> QDCGLPPDVPNAQPALEGRTSFPEDTVITYKCEESFVKIPGEKDSVICLKGSQWSDIEEFCNRSQDCGLPPDVPNAQPALEGRTSFPEDTVITYKCEESFVKIPGEKDSVICLKGSQWSDIEEFCNRSCEVPTRLNSASLKQPYITQNYFPVGTVVEYECRPGYRREPSLS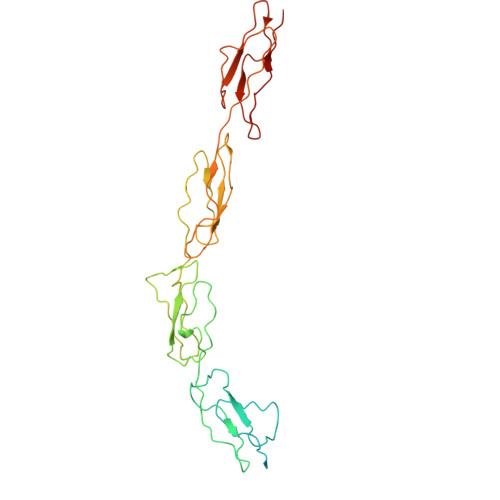PKLTCLQNLKWSTAVEFCKKKSCPNPGEIRNGQIDVPGGILFGATISFSCNTGYKLFGSTSSFCLISGSSVQWSDPLPECREIYCPAPPQIDNGIIQGERDHYGYRQSVTYACNKGFTMIGEHSIYCTVNNDEGEWSGPPPECRG Two glycosyltransferases (GTases), SdgB and SdgA, are responsible for the glycosylation of S. aureus SDR proteins such as ClfA and ClfB. SdgB first appends N-acetyl­glucosamine (GlcNAc) moieties onto serine residues (O-glycosylation) within the SDR domain using uridine diphos­phate N-acetylglucosamine (UDP-GlcNAc) as a donor substrate. The subsequent addition of GlcNAc to the glycoproteins is catalyzed by the second enzyme, SdgA, yielding glycosylated SDR proteins in which each SD repeat is decorated with GlcNAc disaccharide moieties. The glycosylation of SDR proteins mediated by SdgA and SdgB protects SDR proteins from degradation by host proteases, thereby circumventing innate immune attack.

Despite the biological significance of these two glycosyltransferases involved in pathogenicity and avoidance of the host innate immune response, their structures and the molecular basis of their activity have not been investigated. This study reports the crystal structures of SdgB and SdgA from S. aureus as well as multiple structures of SdgB in complex with its substrates (for example UDP, N-acetylglucosamine or SDR peptides), products (glycosylated SDR peptides) or phosphate ions. SdgB undergoes dynamic changes in its structure such as a transition from an open to a closed conformation upon ligand binding and takes diverse forms, both as a homodimer and as a heterodimer with SdgA. We found that SdgB and SdgA have a unique inserted domain, which is used to form a homodimer or heterodimer of SdgB and SdgA.

>SMNYFVGNSLGVNLTGIEKAIINRLNLFKEMGRPAQCVFLSWNRYLYRNAQNYITSSDYINMYDFFQEATYLERNEPFDWLSYWTDECHYTLKHVENSHDFRIYDQERFLMYAHFQDPKYRILDYVNHFDSQRRKVKRDFYDVRGFLSCSRILVDKQQTLCEFFYNPEGDTKLEKYFSYKDGKPEVQKIIVYYANKQYFFNNETELGAFFIKQLYQHGDLFFSDRNVYTAPIFNLTPESIPVVAVLHSTHIKNIDALDSSPFKNVYKAMFENLSRYRAIIVSTEQQKLDVEKRINHTIPVVNIPVGYSETIDTPVQTLDQRSVKLISVARYSPEKQLHQQIELIKRLVSYVPKIELHMYGFGSESKKLNELIQKYGLENHVYLRGFLSNLDQEYSDAYLSLITSNMEGFSLALLESLAHGVPVISYDIKYGPNELITSDFNGYLITKNDEDALFDKVKYVIDHPEVQQRLSKGSLAKAQQYSKASLIKQWDQFVRLILEHHHHHH[2x]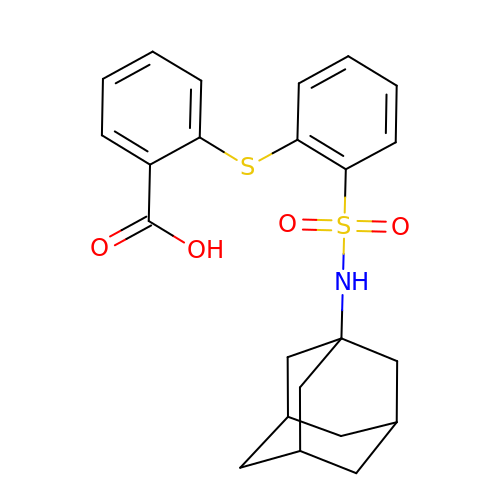2-[(2-{[(3s,5s,7s)-adamantan-1-yl]sulfamoyl}phenyl)sulfanyl]benzoic acid | C23 H25 N O4 S2 | IEUWYSKTODWTNP-FWWHLXPUSA-N>MSLKTLNIYLMRHGKVDAAPGLHGQTDLKVKEAEQQQIAMAWKTKGYDVAGIISSPLSRCHDLAQILAEQQLLPMTT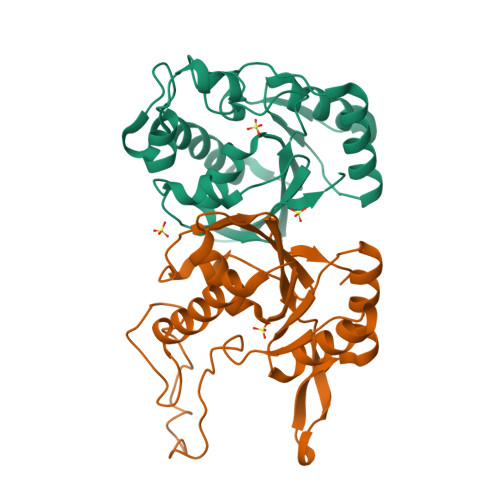EDDLQEMDFGDFDGMPFDLLTEHWKKLDAFWQSPAHHSLPNAESLSTFSQRVSRAWSQIINDINDNLLIVTHGGVIRIILAHVLGVDWRNPQWYSTLAIGNASVTHITITIDDQIYASVRSIGVPLVEEGHHHHHH[2x]> MHHHHHHMQIGWRREGIKYRRNELFLDVLESVNLLMSPQGQVLSAHVSGRVVMKSYLSGMPECKFGMNDKIVIEKQGKGTADETSKSGKQSIAIDDCTFHQCVRLSKFDSERSISFIPPD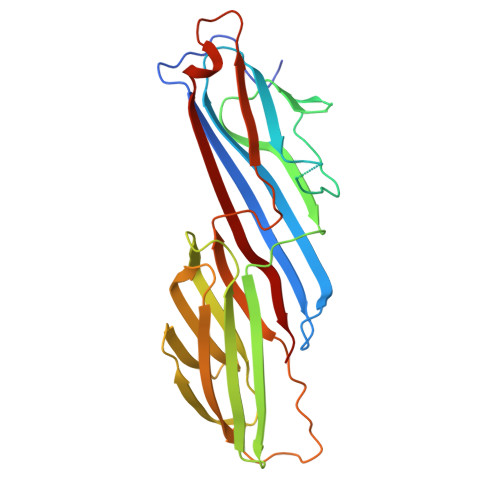GEFELMRYRTTKDIILPFRVIPLVREVGRTKLEVKVVIKSNFKPSLLAQKIEVRIPTPLNTSGVQVICMKGKAKYKASENAIVWKIKRMAGMKESQISAEIELLPTNDKKKWARPPISMNFEVPFAPSGLKVRYLKVFEPKLNYSDHDVIKWVRYIGRSGIYETRC> MAAVILESIFLKRSQQKKKTSPLNFKKRLFLLTVHKLSYYEYDFERGRRGSKKGSIDVEKITCVETVIPEKNPPPERQIPRRGEESSEMEQISIIERFPYPFQVVYDEGPLYVFSPTEELRKRWIHQLKNVIRYNSDLVQKYHPCFWIDGQYLCCSQTAKNAMGCQILENRNGSLKPGSSHRKTKKPLPPTPEEDQILKKPLPPEPTAAPISTTELKKVVALYDYMPMNANDLQLRKGEEYFILEESNLPWWRARDKNGQEGYIPSNYITEAEDSIEMYEWYSKHMTRSQAEQLLKQAGAAGGFIVRDSSKAGKYTVSVFAKSTGEPQGVIRHYVVCSTPQSQYYLAEKHLFSTIPELINYHQHNSAGLISRLKYPVSKQNKNPPPPPGFGYGSWEIDPKDLTFLKELGTGQFGVVKYGKWRGQYDVAIRMIREGSMSEDEFIEEAKVMMNLSHEKLVQLYGVCTKQRPIFIITEYMANGCLL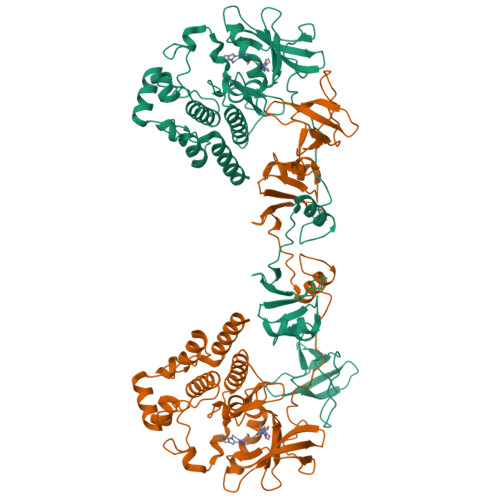NYLREMRHRFQTQQLLEMCKDVCEAMEYLESKQFLHRDLAARNCLVNDQGVVKVSDFGMTRYVLDDEYTSSTGSKFPVKWASPEVLMYSKFSSKSDIWAFGVLMWEIYSLGKMPYERFTNSETAEHIAQGLRLPRPHLASERVYTIMYSCWHEKADERPSFKILLSNILDVMDEES> QGVDQSPKPLIIGPEEDYDPGYFNNESDIIFQDLEKLKSRPAHLGVFLRYIFSQADPSPLLFYLCAEVYQQASPKDSRSLGKDIWNIFLEKNAPLRVKIPEMLQAEIDSRLRNSEDARGVLCEAQEAAMPEIQEQIHDYRTKRTLGLGSLYGENDLLDLDGDPLRERQVAEKQLAALGDILSAYAADRSA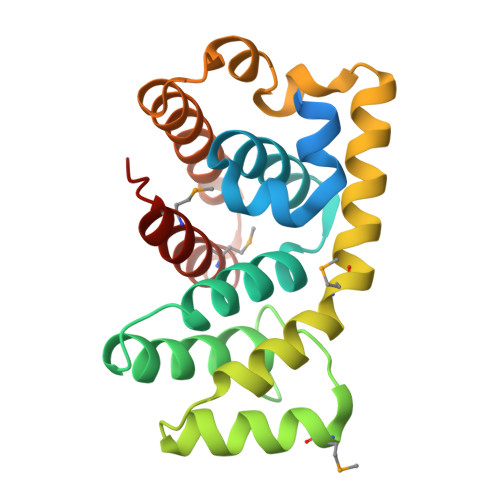PMDFALNTYMSHAGIRLREA2-(imidazo[1,2-a]pyridin-2-yl)-N-phenylacetamide | C15 H13 N3 O | 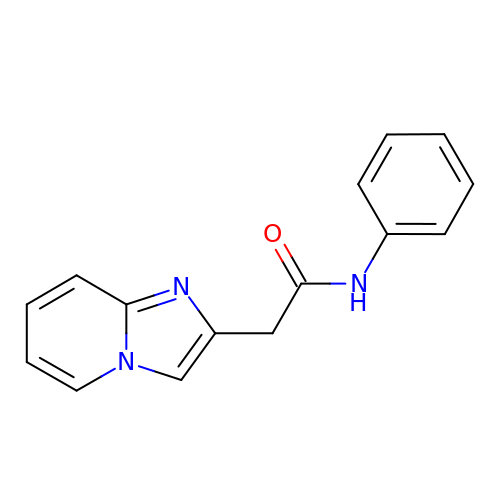NYOYOCWWJBDHMW-UHFFFAOYSA-N>TLLAAITSFGLIGGAYAAEERSYILATASTGGTYYPVGVALATLTKVKLTPSYHFSLSAISSAGSGENVKLMNDNEAQFAILQGLYGAWAWAGEGPYAERQNQLRSVSMLWQNVEHFIVRSDLAPTGTIADLASMKGKKFSIGSKNSGTEFSGRQIMKGVGVDPDTFNLAYLGYGGSASALQNGTIDGMNTPAGVPVGAVTQAFAAMGNDIKILSFTDEQIKQANGNYNLWTKFDIPANTYPGVDKTITTIAQPNFLAVRTDISEEDVYQLTKAMYENLAFLQGIHKATKDMAIEKAIEG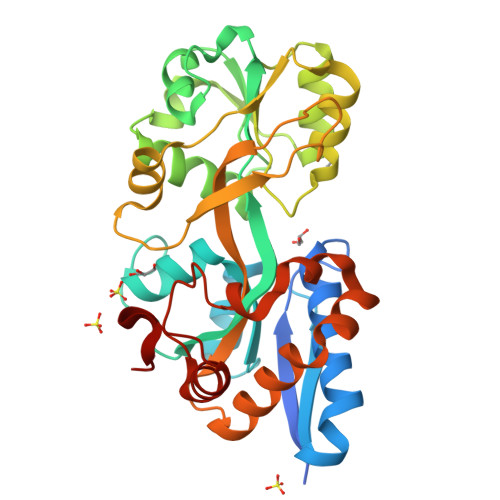LPMPLHAGAARYYQEVGIKIPAHLMPQ[2x]> MKSSDIFFAYRLTPVVFKSRQHDSGVNQYGLKPTNAYDYINPTNLINFGRGTTFDNLGVRRAGRGEIDSSPSHSG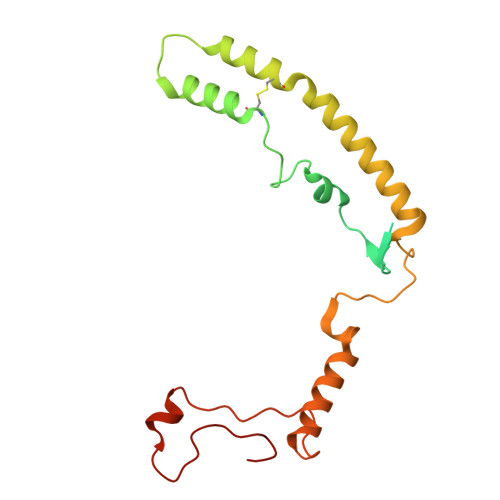SPVFTQAKLIGLSGEEQLTMCQSETMALRLCMAKAGKETCERESRALDSCLGRVGHLRRAMSEACWEFNDWFIQNVSDNHTKPFQHRPHDWRHFYAQEKLVRERQQNGHAYGRRPKQFSFGARYVKTDGYGKRPRLPYNK> MAKSHHHHHHTSTKAERWQARKDLIAKGSNSLYPDAQIAAKRLAANNIAVEKAKLAENVYKTVNPLEATPGVPEGWKDISNDAGALKKYGLDKEVLFDHADTPDFLARVYQPDSAVFGSDMNPTIVFRGSRQPEFFPTKNMADWINNGAQGLGMESDYYKRAVRLGSRLAKSVSKIDIAGHSLGGGLASATSIASGQAGWTFNAAGLHSTTVEKYGGSLLGEADNIQAYRVEGELLTKIQEVNLAEDYKMLKGHIPTLIAKEEISAIMPNAAGVVHDLPGGTGGPLDRHGIGQAIDCIEQQKDEDISIIRSRA;> MDLKPDNYFSGQQLTLARAIENGEVDEVIKLASGTDLNKPGKEDMTLLFWAVMNSINNQKTPERLNVITMLIKAGADPLQPRPQGKNSPAEFVLMADNADWIKAMLNAGLSPNAVDKTFGKPIIFQTLEAKNTKTLQAMLDKGADINITDSLGNTLLIDALDFHSYDHVLLLLERGADPEIKADNGWTMGNQLQRFLDRAKVGSDEYKKLNEIKDVLIQHGGKWPPTPVK

Here, we show that AGE crosslinking is harnessed to activate an antibacterial phospholipase effector protein deployed by the type VI secretion system of Enterobacter cloacae. Endogenous methylglyoxal reacts with a specific arginine-lysine pair to tether the N- and C-terminal α-helices of the phospholipase domain. Substitutions at these positions abrogate both crosslinking and toxic phospholipase activity, but in vitro enzyme function can be restored with an engineered disulfide that covalently links the N- and C-termini. Thus, AGE crosslinking serves as a bona fide post-translation modification to stabilize phospholipase structure.

To identify the Tle modification, we solved the crystal structure of the His6-lipase•∆ss-Tli complex to 1.75 Å resolution using sulfur single-wavelength anomalous diffraction (S-SAD). The lipase domain adopts an α/β-hydrolase fold with a central 7-strand mixed β-sheet surrounded by 13 α-helices. Residues Ser341, Glu393 and His448 (numbered according to full-length Tle) comprise the lipase catalytic triad, with Ser341 projecting from a classical nucleophilic ‘elbow’ that connects β4 to α7. The lipase-immunity protein interface is extensive (~3,900 Å2), corresponding to 14.9% of lipase domain and 17.1% of ∆ss-Tli surface area. The inner helical layer (α8, α10 and α12) of the immunity protein solenoid accounts for most of the contacts with the lipase, though the long loop connecting the 2nd and 3rd ankyrin repeats also forms several hydrogen bonds. Strikingly, lipase helix α6 is pulled away from the main body of the domain through interactions with ∆ss-Tli. Surprisingly, Tle appears to adopt an activated conformation when bound to Tli, because the lipase catalytic triad is exposed to solvent in the crystal structure. The crystal structure also reveals an unusual interaction between the positively charged sidechains of lipase residues Arg180 from helix α1 and Lys461 in helix α13. Fo-Fc difference maps show continuous electron density between these sidechains, suggesting that the residues are covalently linked. The +36 Da mass shift observed in the modified lipase domain is consistent with a methylglyoxal-derived imidazolium crosslink (MODIC), and MODIC fits well into the electron density bridging Arg180 and Lys461.>[2x]GAMEPSLYTVKAILILDNDGDRLFAKYYDDTYPSVKEQKAFEKNIFNKTHRTDSEIALLEGLTVVYKSSIDLYFYVIGSSY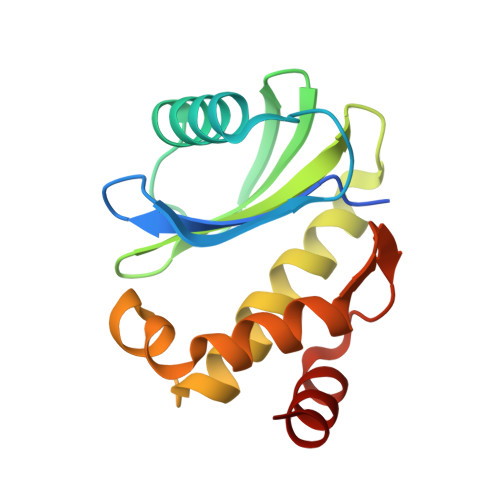ENELMLMAVLNCLFDSLSQMLRKNVEKRALLENMEGLFLAVDEIVDGGVILESDPQQVVHRVALRG>SRASEHRNEKGERISMINPRVVLDENGISHRSRYFIMLCDNETAIAHAKKTSIWAVKKDSSKRISDAYKKASVYFIFVAQQTYNALGYAQVVSDLN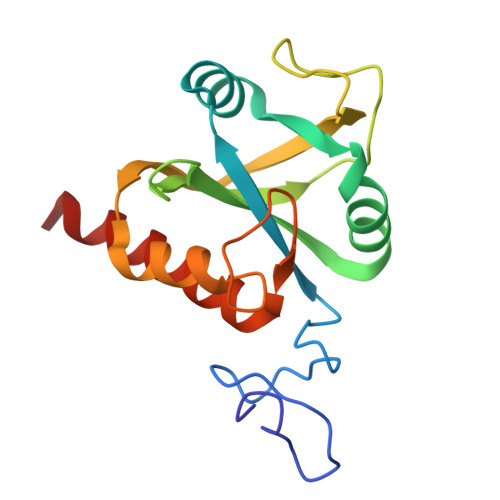STELPFWSDSSHAGGVRIKWIKTCNLFSAEISEIVSHMDHGSEARDGMEMMYDEGSRLCTLINYAIMKRIGRDR[4x]> MSKKHPIISVTGSSGAGTSTVKHTFDQIFRREGVKAVSIEGDAFHRFNRADMKAELDRRYAAGDATFSHFSYEANELKELERVFREYGETGQGRTRTYVHDDAEAARTGVAPGNFTDWRDFDSDSHLLFYEGLHGAVVNSEVNIAGLADLKIGVVPVINLEWIQKIHRDRATRGYTTEAVTDVILRRMHAYVHCIVPQFSQTDINFQR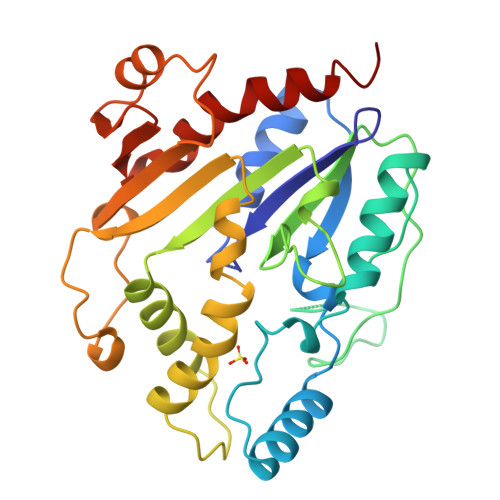VPVVDTSNPFIARWIPTADESVVVIRFRNPRGIDFPYLTSMIHGSWMSRANSIVVPGNKLDLAMQLILTPLIDRVVRESKVA> XK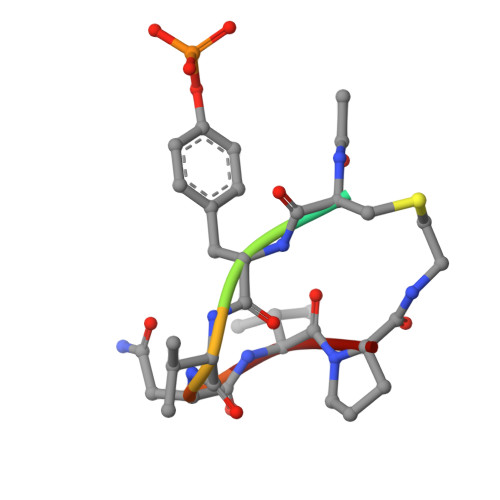YVNVP>MGILQANRVLLSRLLPGVEPEGLTVRHGQFHQVVIASDRVVCLPRTAAAAARLPRRAAVMRVLAGLDLGCRTPRPLCEGSAEGAVELPFLVLSRVPGAPLEADALEDSKVAEVVAAQYVTLLSGLASAGADEKVRAALPAPQGRWRQFAADVRAELFPLMSDGGCRQAERELAALDSLPDITEAVVHGNLGAENVLWVRDDGLPRLSGVIDWDEVSIGDPAEDLAAIGAGYGKDFLDQVLTLGGWSDRRMATRIATIRATFALQQALSACRDGDEEELADGLTGYR[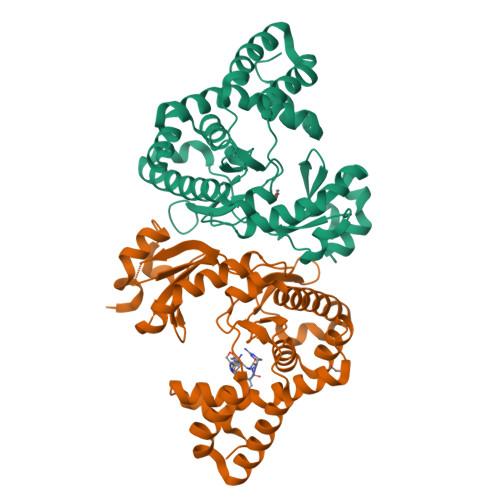2x]PYP is a highly soluble globular protein from the PAS domain superfamily. Apo-PYP, as expressed in cells, forms a covalent complex with the chromophore, p-coumaric acid (pCA), a process that is analogous to covalent drug binding. While not a drug target in the conventional sense, it shares chemical characteristics with common covalent drug targets, especially those with reactive cysteines. Utilizing this spectrometer, we employed photoactive yellow protein (PYP) and its covalently attached chromophore p-coumaric acid (pCA) as a representative framework for many cysteine-based covalent inhibitors.

Each nitrile-containing PYP variant was previously characterized in the holo-form (covalently attached to pCA) via X-ray crystallography to high-resolution (<1.2 Å), where the nitriles adopt a single, well-defined orientation at each site. The absence of the chromophore and nitrile labels did not result in any major conformational changes in the protein structure, except for a lack of density in the disordered loop region (residues 16–20), which is located more than 20 Å from the chromophore pocket. However, when apo-PYP nitrile frequencies were compared to previous measurements conducted on the purified holo-PYP (with pCA covalently attached), significant differences in peak frequency were noted for variants F92oCNF and F96oCNF. 24 The current simulations in the absence of the chromophore significantly favor decreased hydrogen bonding of the nitrile to T90 in apo-F92oCNF, consistent with the IR measurements showing a blue shift upon chromophore incorporation. In the case of F92oCNF, chromophore incorporation appears to increase its potential to form a hydrogen bond with T90, whereas in the apo state, it remains largely isolated from such interactions. Structurally, the crystallographic data seem to suggest a slight reorientation of F96 toward the empty chromophore pocket and slight increase in hydrogen bonding population. Additionally, AMOEBA simulations reveal a small increase in hydrogen-bonded population (nitrile-to-solvent) for the apo-F96oCNF variant upon pCA binding. However, the small but definite change in solvent hydrogen bonding to the nitrile in F96oCNF presents a reasonable explanation for the smaller blue shift undergone by the nitrile upon pCA binding.

>[2x]MEHVAFGSEDIENTLAKMDDGQLDGLAFGAIQLDGDGNILQYNAAEGDITGRDPKQVIGKNFFKDVAPCTDSPEFYGKFKEGVASGNLNTMFEYTFDYQMTPTKVKVHMKKALSGDSYWVFVKRV>DDGICKSSDCIKSAARLIQNMDATTEPCTDFFKYACGGWLKRNVIPETSSRYGNFDILRDELEVVLKDVLQEPKTEDIVAVQKAKALYRSCINESAIDSRGGEPLLKLLPDIYGWPVATENWEQKYGASWTAEKAIAQLNSKYGKKVLINLFVGTDDKNSVNHVIHIDQPRLGLPSRDYYECTGIYKEACTAYVDFMISVARLIRQEERLPIDENQLALEMNKVMELEKEIANATAKPEDRNDPMLLYNKMTLAQIQNNFSLEINGKPFSWLNFTNEIMSTVNISITNEEDVVVYAPEYLTKLKPILTKYSARDLQNLMSWRFIMDLVSSLSRTYKESRNAFRKALYGTTSETATWRRCANYVNGNMENAVGRLYVEAAFAGESKHVVEDLIAQIREVFIQTLDDLTWMDAETKKRAEEKALAIKERIGYPDDIVSNDNKLNNEYLELNYKEDEYFENIIQNLKFSQSKQLKKLREKVDKDEWISGAAVVNAFYSSGRNQIVFPAGILQPPFFSAQQSNSLNYGGIGMVIGHEITHGFDDNGRNFNKDGDLVDWWTQQSASNFKEQSQCMVYQYGNFSWDLAGGQHLNGINTLGENIADNGGLGQAYRAYQNYIKKNGEEKLLPGLDLNHKQLFFLNFAQVWCGTYRPEYAVNSIKTDVHSPGNFRIIGTLQNSAEFSEAFHCRKNSYMNPEKKCRVW[2x]

Neprilysin, also called neutral endopeptidase, enkephalinase, or atriopeptidase, is a zinc dependent type II integral membrane peptidase belonging to the M13 family. It degrades a variety of vasoactive peptides such as atrial natriuretic peptide, brain natriuretic peptide, bradykinin, adrenomedullin and endothelin-15. The extracellular domain of NEP is comprised of two largely α-helical subdomains, with domain 1 predominantly containing C-terminal residues while domain 2 is formed mainly from the N-terminal half of the protein. The two domains are arranged to harbor a large cavity in the center that contains the catalytic machinery which is formed by residues from domain 1.

NEP in complex with LBQ657 crystallized in the orthorhombic space group P212121 with two copies in the asymmetric unit diffracting to 2.0 Å resolution. LBQ657 is bound to the active site of NEP by an intricate network of interactions that involves all functional groups of the compound giving rise to the high inhibitory potency of 5 nM12. In the crystal structure, the catalytic zinc atom of NEP is ligated by the side chains of residues His583 (2.0 Å), His587 (1.9 Å) and Glu646 (2.0 Å) with the fourth coordination provided by the carboxylate oxygen adjacent to the P1 methyl of the compound (2.0 Å). The methyl group of LBQ657 is pointing towards the shallow S1 pocket making hydrophobic interactions with Phe544. The backbone amide of LBQ657 forms H-bonding interactions with the side chains of Asn542 and Arg717. It places the carboxylic acid in an ideal position for optimal interaction with Arg102 and Arg110, unique for LBQ657. The P1’ biphenyl of LBQ657 binds deeply in the S1’ subsite of NEP, inducing conformational changes for optimal hydrophobic interactions. When comparing our co-crystal structure to one with a compound harboring a benzyl in P1’8, an analogous induced fit of Trp693 towards the S2’ subsite is observed, which in turn leads to a conformational change of Phe106. In NEP the space occupied by the new orientation of Trp693 is available because the adjacent Gly714 does not project a sidechain towards this area. The residues corresponding to Gly714 are Ser735 (ECE-1)13 and Leu744 (NEP2) and their side chains will impose steric constraints to the conformational change of Trp714 (ECE-1) and Trp723 (NEP2), respectively.>[4x]HTRMFSVWVNGVDQGDGQNVYIRTPPNTDPIKDLASPALACNVKGGEPVPQFVSASAGDKLTFEWYRVKRGDDIIDPSHSGPITTWIAAFTSPTMDGTGPVWSKI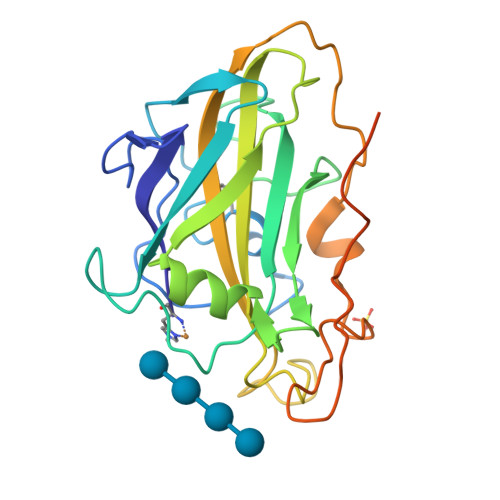HEEGYDASTKSWAVDKLIANKGMWDFTLPSQLKPGKYMLRQEIVAHHESDATFDKNPKRGAQFYPSCVQVDVKGVGGDAVPDQAFDFNKGYKYSDPGIAFDMYTDFDSYPIPGPPVWDAQDEGCCFIDGVDTTSVKEVVKQIICVLK> MSEFLTPERTVYDSGVQFLRPKSLDEFIGQENVKKKLSLALEAAKMRGEVLDHVLLAGPPGLGKTTLAHIIASELQTNIHVTSGPVLVKQGDMAAILTSLERGDVLFIDEIHRLNKAVEELLYSAIEDFQIDIMIGKGPSAKSIRIDIQPFTLVGATTRSGLLSSPLRSRFGII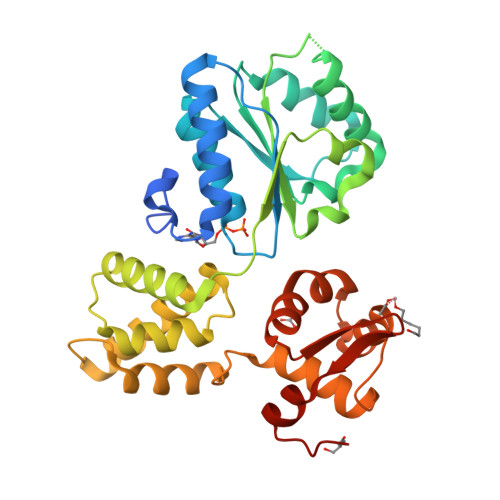LELDFYTVKELKEIIKRAASLMDVEIEDAAAEMIAKRSRGTPRIAIRLTKRVRDMLTVVKADRINTDIVLKTMEVLNIDDEGLDEFDRKILKTIIEIYRGGPVGLNALAASLGVEADTLSEVYEPYLLQAGFLARTPRGRIVTEKAYKHLKYEVPENRLF>[2x]MDIISVALKRHSTKAFDASKKLTPEQAEQIKTLLQYSPSSTNS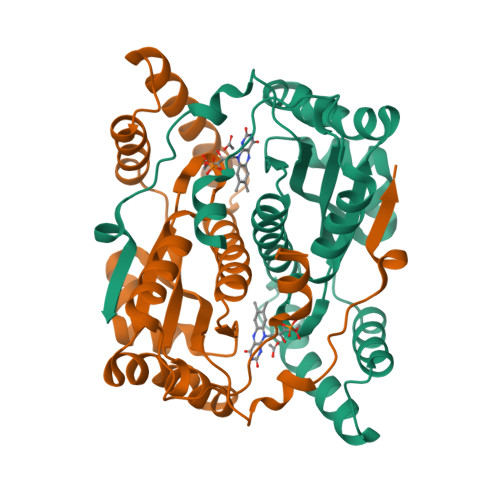QPWHFIVASTEEGKARVAKSAAGNYVFNERKMLDASHVVVFCAKTAMDDVWLKLVVDQEDADGRFATPEAKAANDKGRKFFADMHRKDLHDDAEWMAKQVYLNVGNFLLGVAALGLDAVPIEGFDAAILDAEFGLKEKGYTSLVVVPVGHHSVEDFNATLPKSRLPQNITLTEV> AGVMTGAKFTQIQFGMTRQQVLDIAGAENCETGGSFGDSIHCRGHAAGDYAAYATFGFTSAAADAKVDSKSQEKLLAPSAPTLTLAKFNQVTVGMTRAQVLATVGQGSCTTWSEYYPAYPSTAGVTLSLSCFDVDGYSSTGF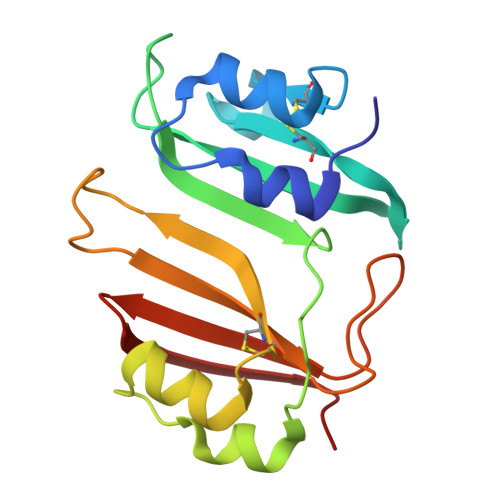YRGSAHLWFTDGVLQGKRQWDLV Enhanced ABA levels elicited in response to drought are perceived by the PYR/PYL/RCAR family of ABA receptors and the clade A subfamily of protein phosphatases type 2C (PP2Cs), which act as necessary ABA co-receptors in ternary complexes. In the resting state, PYLR/PYL/RCAR receptors display an open ABA binding cavity flanked by two highly conserved loops, named as gate/CL2/β3-β4 loop and latch/CL3/β5-β6 loop. Specifically, both gate and latch loops define a surface that enables the receptor to dock into the PP2C active site. The formation of receptor-ABA-phosphatase complexes causes the dissociation of different PP2C-SnRK2 complexes and abolishes PP2C-mediated inhibition of the SnRK2s, triggering ABA response.

We reasoned that swapping the positions of the SO2 and CH2 moieties in the SB linker might contribute to fill this cavity by promoting the formation of a hydrogen bond between the SO2 moiety of the agonist and the Lys88 side chain, increasing ligand activity. We, therefore, synthesized two new compounds incorporating the above swap, iSB07 and iSB09 (“inverted SB”). Compared to iSB07, iSB09 contains a larger alkyl group (ethyl versus methyl) at the dihydroquinoline ring that might increase ligand activity through interaction with the 3′ tunnel for SB-01. To gain insight into the structural basis of iSB agonist activity, we solved the crystal structures of CsPYL1-iSB07-HAB1, CsPYL1-iSB09-HAB1, CsPYL15m-iSB07-HAB1, and CsPYL15m-iSB09-HAB1. Consistent with our docking predictions, both iSB07 and iSB09 complexes display the hydrogen bond network to conform the Trp lock and the compounds show a hydrogen bond between the oxygen of the SO2 moiety and side-chain NH3+ of Lys88 and, unexpectedly, an additional one to the guanidinium moiety of Arg108 side chain. In addition, iSB09 structures reveal that iSB09’s ethyl group, compared to iSB07’s methyl group, increases the number of hydrophobic contacts at the 3′ tunnel without distorting the conformation of the gate. Specifically, the structure of the sulfonamide linker displays a more likely and relaxed conformation (in terms of the torsion angles) for agonists in the ligand-binding pocket of CsPYL15m than in CsPYL1. We also conducted isothermal titration calorimetry (ITC) experiments comparing ABA-CsPYL1-HAB1 and iSB09-CsPYL15m-HAB1 binding reactions. These experiments show a similar Kd (dissociation constant) for ABA and iSB09 binding in these ternary complexes, which suggests that the combination iSB09-CsPYL15m-HAB1 matches the affinity of ABA binding in the ABA-CsPYL1-HAB1 complex. Using the available structural information, we have designed the synthetic CsPYL15m receptor to enhance the effect of iSB09, thus obtaining an optimized receptor-ligand pair, in other words, a receptor ad hoc to bind iSB09.

> MNNNKAEADTSSSMADPETRPTYTTHHLAIPSGVTQDEFDELKQSVVEFHTYQLSQNQCSSLLAQRIRAPNDVVWSIVRRFDQPQTYKHFIKSCSVSDNFTMAVGSTRDVNLISGLPAATSTERLDILDDDRQVLGISIIGGEHRLRNYRSVISVHGFNRDGAICTVALESYVVDVPEGNTEEDTRLFADTVVKLNLQKLVSVAESQVI;> RSVYELDCIPLWGTVSIQGNRSEMEDAFAVSPHFLKLPIKMLMGDHEGMSPSLTHLTGHFFGVYDGHGGHKVADYCRDRLHFALAEEIERIKDELCKRNTGEGRQVQWDKVFTSCFLTVDGEIEGKIGRAVVGSSDKVLEAVASETVGSTAVVALVCSSHIVVSNCGDSRAVLFRGKEAMPLSVDHKPDREDEYARIENAGGKVIQWQGARVFGVLAMSRSIGDRYLKPYVIPEPEVTFMPRSREDECLILASDGLWDVMNNQEVCEIARRRILMWHKKNGAPPLAERGKGIDPACQAAADYLSMLALQKGSKDNISIIVIDLKAQRKFKTRT>GFDFAVIKELKTAASQYGATAPYTLAIVESVADNWLTPTDWNTLVRAVLSGGDHLLWKSEFFENCRDTAKRNQQAGNGWDFDMLTGSGNYSSTDAQMQYDPGLFAQIQAAATKAWRKLPVKGDPGASLTGVKQGPDEPFADFVHRL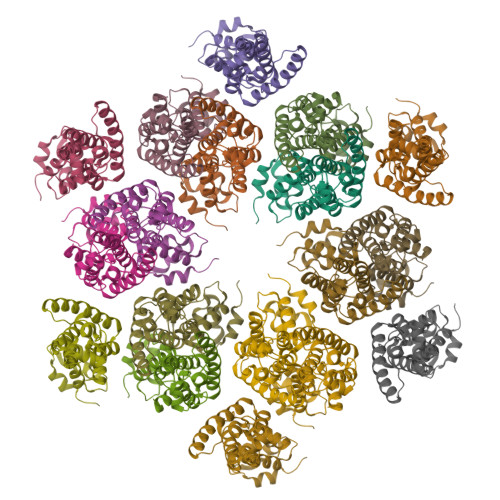ITTAGRIFGSAEAGVDYVKQLAYENANPACQAAIRPYRKKTDLTGYIRLCSDIG[3x]> SESQEDIIR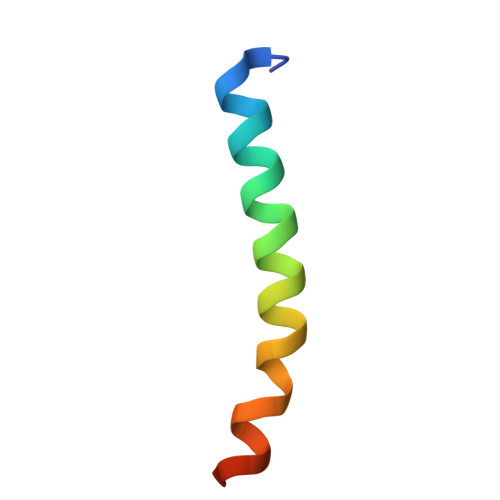NIARHLAQVGDSMDRSIPPGLVNGL> MGGGEVKMMSLLEEMKGIYSKKGGKVKPFEKFEGELKEGYRFEY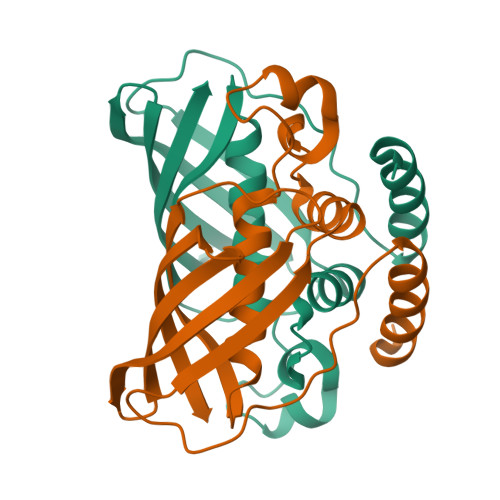EKKLCEIDVAMFGLISGDLNPVHFDEDFASKTRFGGRVVHGMLTTSLVSAAVARLPGTVVLLEQSFRYTSPVRIGDVVRVEGVVSGVEKNRYTIDVKCYTGDKVVAEGVVKVLIW N-[(3R)-3-(cyanomethyl)-1-methyl-2-oxo-2,3-dihydro-1H-indol-5-yl]acetamide 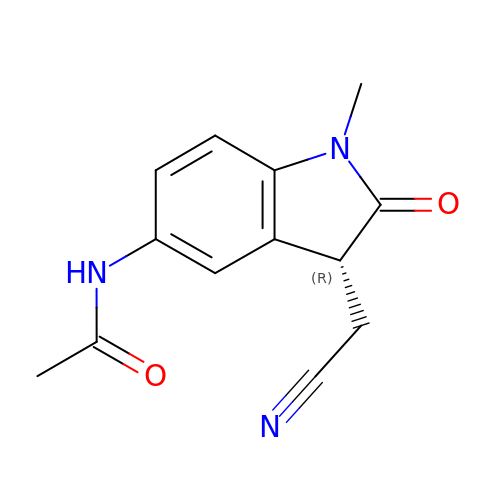| C13 H13 N3 O2 | PFJVUECMVVMLTI-SNVBAGLBSA-N> MIIERLVGNLRDLNPLDFSVDHVDLEWFETRKKIARFKTRQGKDIAIRLKDAPKLGLSQGDILFKEEKEIIAVNILDSEVIHIQAKSVAEV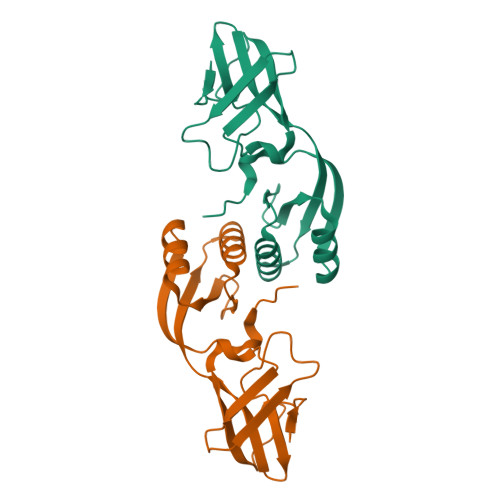AKICYEIGNRHAALYYGESQFEFKTPFEKPTLALLEKLGVQNRVLSSKLDSKERLTVSMPHSEPNFKVSLASDFKVVVK PARA-TOLUENE SULFONATE | C7 H8 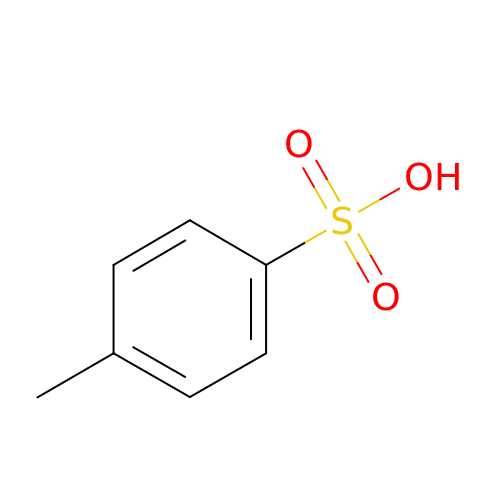O3 S | JOXIMZWYDAKGHI-UHFFFAOYSA-N> HPETLVKVKDAEDQLGARVGYIELDLNSGKILES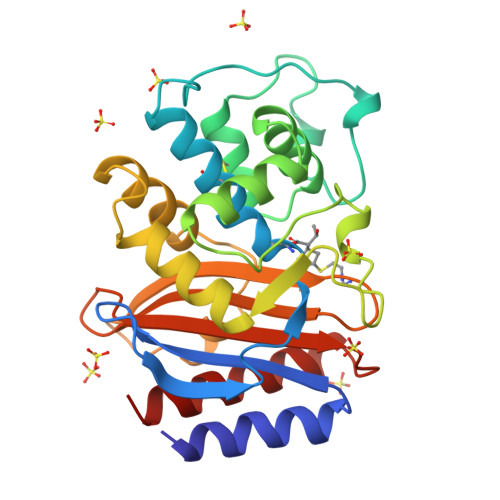FRPEERFPMMSTFKVLLCGAVLSRIDAGQEQLGRRIHYSQNDLVEYSPVTEKHLTDGMTVRELCSAAITMSDNTAANLLLTTIGGPKELTAFLHNMGDHVTRLDRWEPELNEAIPNDERDTTMPVAMATTLRKLLTGELLTLASRQQLIDWMEADKVAGPLLRSALPAGWFIADKSGAGERGSRGIIAALGPDGKPSRIVVIYTTGSQATMDERNRQIAEIGASLIKHW> MAYIKRVIIKGFKTYRNETIIDNFSPHQNVIIGSNGSGKSNFFAAIRFVLSDDYSNLKREERQGLIHQGSGGSVMSASVEIVFHDPDHSMILPSGVLSRGDDEVTIRRTVGLKKDDYQLNDRNVTKGDIVRMLETAGFSMNNPYNIVPQGKIVALTNAKDKERLQLLEDVVGAKSFEVKL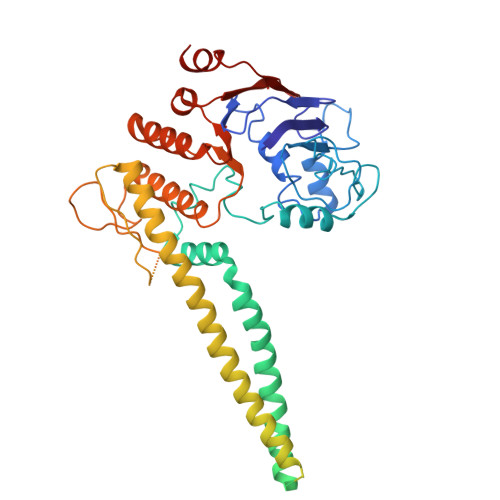KASLKKMEETEQKKIQINKEMGELNSKLSEMEQERKELEKYNELERNRKIYQFTLYDRELNEVINQMERLDGDYNNTVYSSESSKHPTSLVPRGSDITSDQLLQRLNDMNTEISGLKNVNKRAFENFKKFNERRKDLAERASELDESKDSIQDLIVKLKQQKVNAVDSTFQKVSENFEAVFERLVPRGTAKLIIHRKNDNANDHDESIDVDMDAESNESQNGKDSEIMYTGVSISVSFNSKQNEQLHVEQLSGGQKTVCAIALILAIQMVDPASFYLFDEIDACLDKQYRTAVATLLKELSKNAQFICTTFRTDMLQVADKFFRVKYECKISTVIEVNREEAIGFIRGSNKFAEV>[4x]MRGSHHHHHHGMASMPLHHLTRFPRLEFIGAPTPLEYLPRLSDYLGREIYIKRDDVTPIAMGGNKLRKLEFLVADALREGADTLITAGAIQSNHVRQTAAVAAKLGLHCVALLENPIGTTAENYLTNGNRLLLDLFNTQIEMCDALTDPDAQLQTLATRIEAQGFRPYVIPVGGSSALGAMGYVESALEIAQQCEEVVGLSSVVVASGSAGTHAGLAVGLEHLMPDVELIGVTVSRSVAEQKPKVIALQQAIAGQLALTATADIHLWDDYFAPGYGVPNDAGMEAVKLLASLEGVLLDPVYTGKAMAGLIDGISQKRFNDDGPILFIHTGGAPALFAYHPHV

D-cysteine (D-Cys) moieties are found in firefly luciferin, semisynthetic cephalosporin MT141 and malformin A. D-cysteine desulfhydrase (DCyD) is suggested to take part in the catabolic degradation of D-Cys and D-Cys-containing toxic compounds. The polypeptide fold of StDCyD is similar to those of other fold type II PLP-dependent enzymes and consists of a small domain (residues 48–161) and a large domain (residues 1–47 and 162–328). As in other PLP-dependent fold type II enzymes, the active site is situated in a large crevice between the two domains. StDCyD is specific for D-Cys and βCDA, and shows no activity with ACC, although it shares significant sequence identity with ACCDs.

Structures of two distinct crystal forms of recombinant StDCyD were determined by the molecular replacement method. Apart from the unliganded forms, structures of nine enzyme-ligand complexes have also been determined in crystal form I. In all the eleven structures of form I, besides the hexa-histidine tag, six residues at the N-terminus in chains B and C did not have well-defined electron density and hence have not been included in the final model. All the residues of A and D chains were in good electron density. In the form I native structure, 97.1% and 99.7% were in the most favored and allowed regions, respectively, of the Ramachandran plot. In the form I structure, there are two dimers (AB and CD) and in form II structure, there are four dimers (AB, CD, EF and GH) in the asymmetric unit that are similar to the dimeric organization found in other fold type II PLP-dependent enzymes. Electron density map of unliganded StDCyD revealed a significant patch of density with tetrahedral geometry at the active site that could be interpreted as a sulphate (in form I crystal structure) or a phosphate (in form II crystal structure). Form I crystals were obtained in a condition which had sulphate while conditions for obtaining form II had phosphate ions. These ions could be refined to reasonable B factors that were close to those of the surrounding atoms. PLP is bound by a Schiff base linkage to Lys51. The PLP phosphate is held by hydrogen bonding with main chain nitrogen atoms of residues Gly194, Ser195, Ala196, Gly197 and Thr198.> QGDITHMVKLGKLQYSMDYDFQKGELTVNVIQAADLPGMDMSGTSDPYVKVYLMPDKKKKFETKVHRKTLNPVFNESFTFKNVPYADITGKTLIFAIYDFDRFSKHDQIGQVQVPMNSIDLGSVIE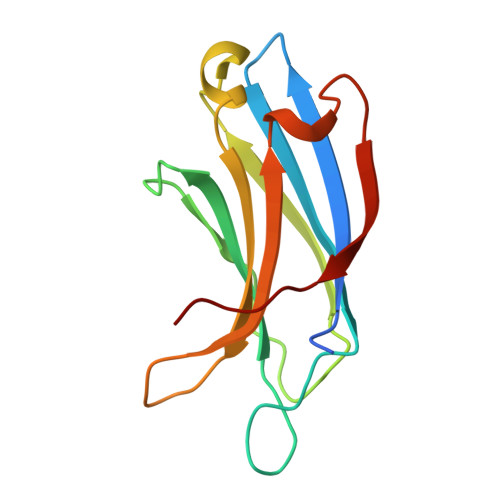EWRDLTSPDN> MAEIGTGFPFDPHYVEVLGERMHYVDVGPRDGTPVLFLHGNPTSSYVWRNIIPHVAPTHRCIAPDLIGMGKSDKPDLGYFFDDHVRFMDAFIEALGLEEVVLV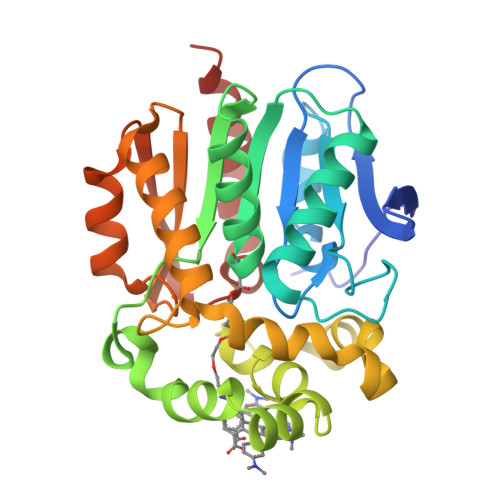IHDWGSALGFHWAKRNPERVKGIAFMEFIRPIPTWDEWPEFARETFQAFRTTDVGRKLIIDQNVFIEGTLPMGVVRPLTEVEMDHYREPFLNPVDREPLWRFPNELPIAGEPANIVALVEEYMDWLHQSPVPKLLFWGTPGVLIPPAEAARLAKSLPNCKAVDIGPGLNLLQEDNPDLIGSEIARWLSTLEISG> KIFKPEELRQALMPTLEALYRQDPESLPFRQPVDPQLLGIPDYFDIVKSPMDLSTIKRKLDTGQYQEPWQYVDDIWLMFNNAWLYNRKTSRVYKYCSKLSEVFEQEIDPVMQSLGYCCGRKLGELFVECTECGRKMHQICVLHHEIIWPAGFVCDGCLKKS;> AGKAFKPEELRQALMPTLEALYRQDPESLPFRQPVDPQLLGIPDYFDIVKSPMDLSTIKRKLDTGQYQEPWQYVDDIWLMFNNAWLYNRKTSAVYKYCSKLSEVFEQEIDPVMQSLGYCCGRKLGELFVECTECGRKMHQICVLH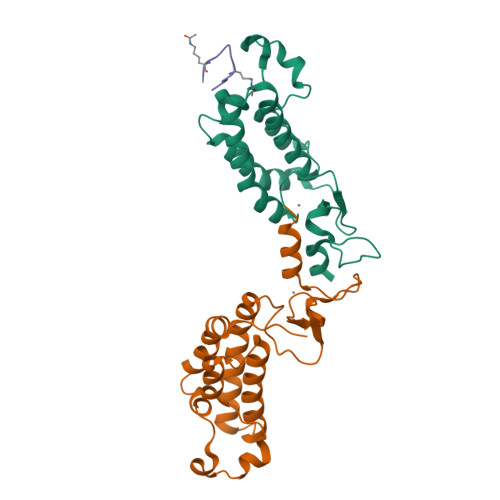HEIIWPAGFVCDGCLKKSARTRK;> GLGKGGAKA>[2x]MKHHHHHHHHGGLVPRGSHGGSEFMTTGLSTAGAQDIGRSSVRPYLEECTRRFQEMFDRHVVTRPTKVELTDAELREVIDDCNAAVAPLGKTVSDERWISYVGVVLWSQSPRHIKDMEAFKAVCVLNCVTFVWDDMDPALHDFGLFLPQLRKICEKYYGPEDAEVAYEAARAFVTSDHMFRDSPIKAALCTTSPEQYFRFRVTDIGVDFWMKMSYPIYRHPEFTEHA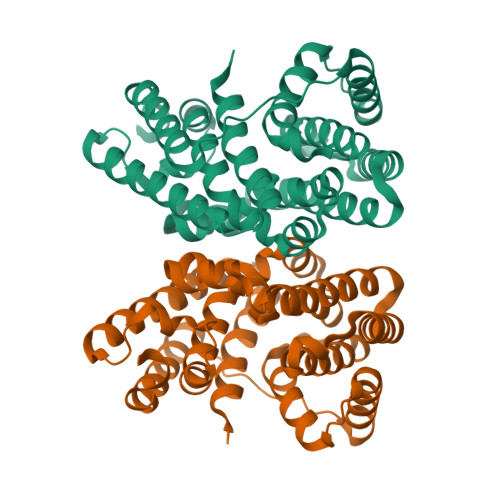KTSLAARMTTRGLTIVNDFYSYDREVSLGQITNCFRLCDVSDETAFKEFFQARLDDMIEDIECIKAFDQLTQDVFLDLIYGNFVWTTSNKRYKTAVNDVNSRIQ[5-hydroxy-6-methyl-4-({[(4E)-3-oxo-1,2-oxazolidin-4-ylidene]amino}methyl)pyridin-3-yl]methyl dihydrogen 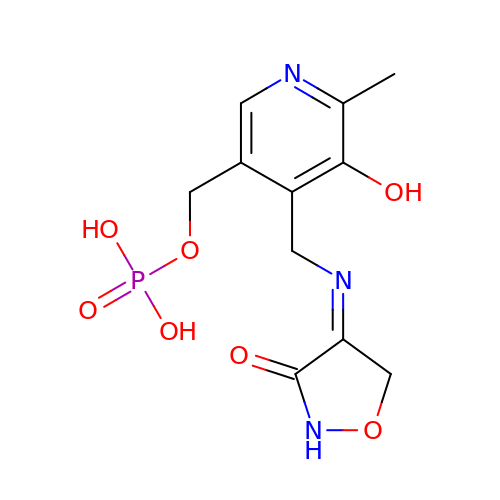phosphate | C11 H14 N3 O7 P | KFCQHWOGBVCKHR-UKTHLTGXSA-N>[2x]MGSSHHHHHHSQDPGHKPEPTDEEWELIKTVTEAHVATNAQGSHWKQKRKFLPEDIGQAPIVNAPEGGKVDLEAFSHFTKIITPAITRVVDFAKKLPMFCELPCEDQIILLKGCCMEIMSLRAAVRYDPESETLTLNGEMAVTRGQLKNGGLGVVSDAIFRLGMSLSSFNLDDTEVALLQA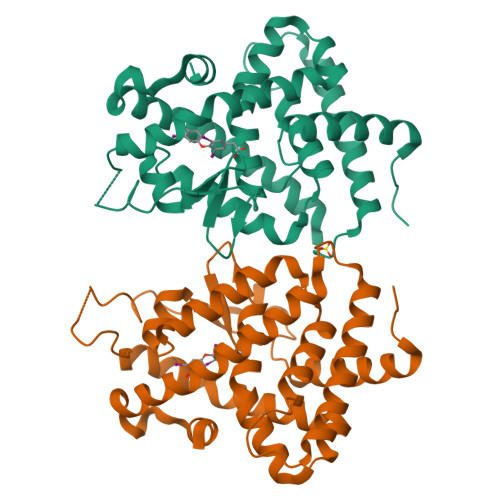VLLMSSDRPGLACVERIEKYQDSFLLAFEHYINYRKHHVTHFWPKLLMKVTDLRMIGACHASRFLHMKVECPTELFPPLFLEVFE Pamamycin 607 | C35 H61 N O7 | 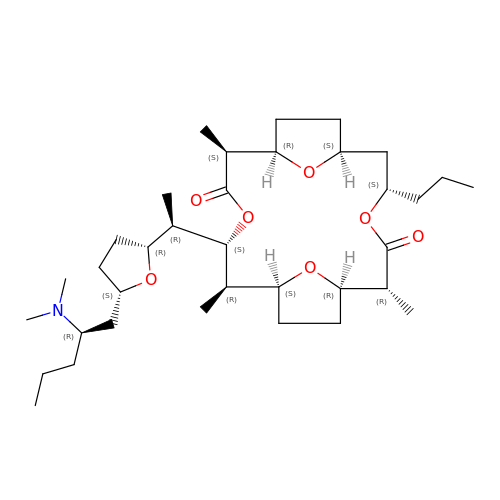AHOIPAFUOXGGQB-IKNPUDIKSA-N(2R)-2-butyloxirane | C6 H12 O | 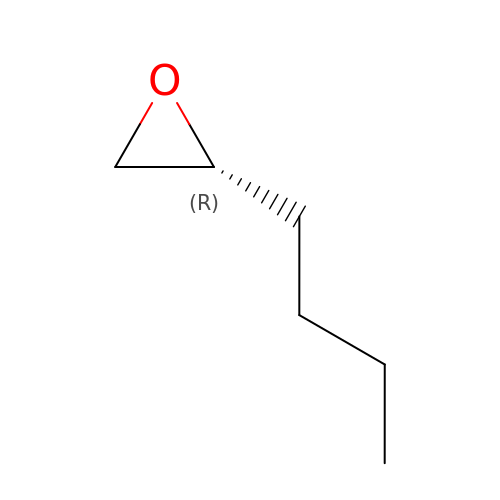WHNBDXQTMPYBAT-ZCFIWIBFSA-N> SKFWEGVLRVLNQISGTLSVIPGPVGTIS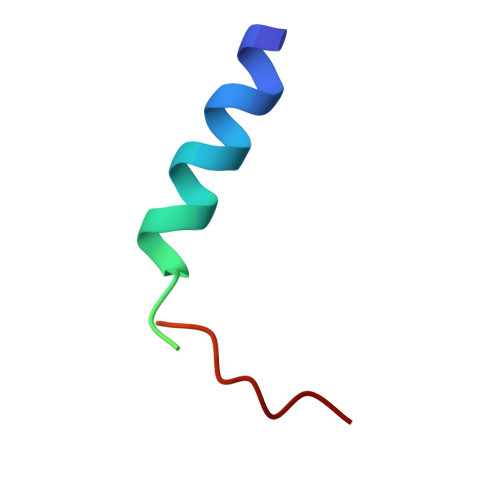AGVHQLTGMYM>[4x]GSHMASNPISEEMNLKILAYLGTKQGAKAVHI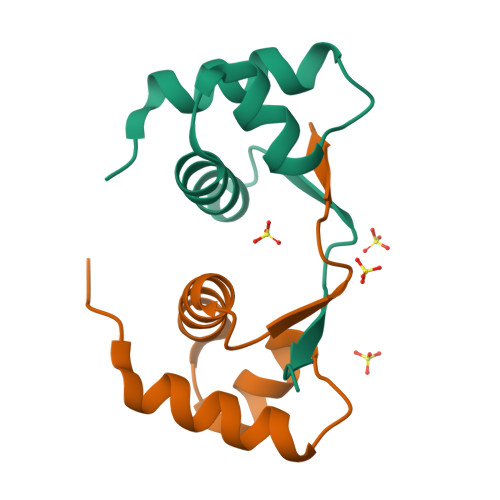AQSLGAQRSEVNRHLYRMSEDGRVRKHPQHPVWYLPA O-(5-methyl-2-nitrophenyl)-D-tyrosinamide | C16 H17 N3 O4 | 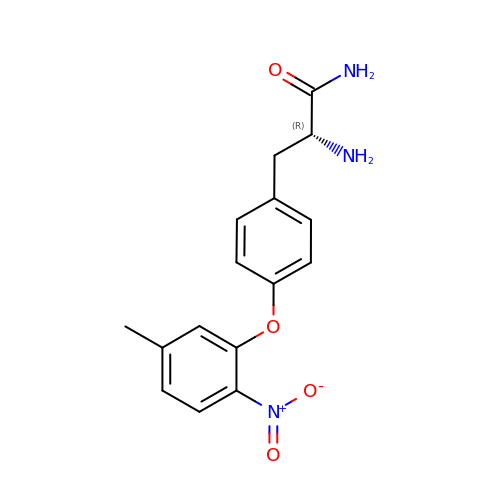YQBKHPZUMXXXFB-CYBMUJFWSA-N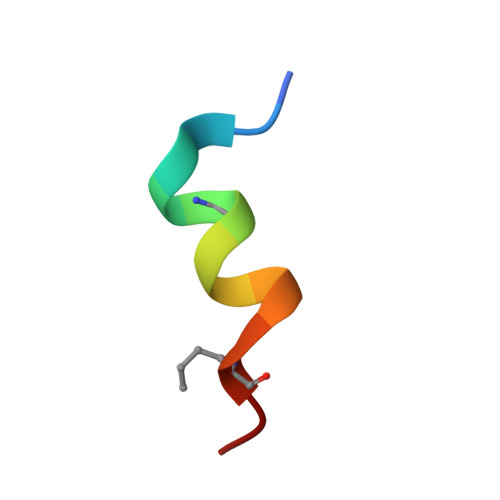> KETAASKFERQHLDS> DIHM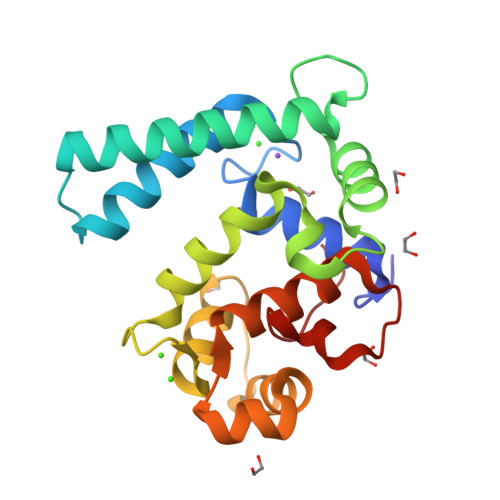AYSWDNRVKYVVRYMYDIDNNGYLDKNDFECLALRNTLIEGRGEFNSDAYANNQKIMSNLWNEIAELADFNKDGQVTVDEFKQAVKNLCCGKSFDGFPPCFKTVIGRLFKTIDINGDGLVGVDEYRLDCISRSAFSSVKEIDDAYAKLCTDDDKKAGGISLNRYQELYAQFISNPDEKCNAVYLFGPLKEVQ> MGSSHHHHHHHSSGRENLYFQGHMEGVRWAFSCGTWLPSRAEWLLAVRSIQPEEKERIGQFVFARDAKAAMAGRLMIRKLVAEKLNIPWNHIRLQRTAKGKPVLAKDSSNPYPNFNFNISHQGDYAVLAAEPELQVGIDIMKTSFPGRGSIPEFFHIMKRKFTNKEWETIRSFKDEWTQLDMFYRNWALKESFIKAIGVGLGFELQRLEFDLSPLNLDIGQVYKETRLFLDGEEEKEWAFEESKIDEHHFVAVALRKPDGSRHQDVPSQDDSKPTQRQFTILNFNDLMSSAVPMTPEDPSFWDCFCFTEEIPIRNGTKS;> GTRDRDSQRDLVEAVAHILGIRDLAAVNLDSSLADLGLDALMSVEVRQTLERELNLVLSVREVRQLTLRKLQELSSKADEASELACPTPKE

The posttranslational modification of a conserved serine residue in carrier proteins with a phosphopantetheinyl moiety transferred from coenzyme A through the enzyme phosphopantetheinyl transferase (PPT) is vital to all living organisms. Molecular cloning and biochemical characterization of human PPT revealed that this cytosolic enzyme is a Mg2+-requiring monomeric enzyme that exhibits a broad acceptor substrate specificity. Whereas microbial genomes contain more than one PPT, only one PPT has been identified in mammals. This enzyme exhibits a broad substrate specificity and is able to phosphopantetheinylate the ACP components of the cytosolic and the mitochondrial FAS systems, as well as aminoadipate semialdehyde dehydrogenase, the human ortholog to the yeast lys5 gene. Human phosphopantetheinyl transferase exhibits an α/β fold and 2-fold pseudosymmetry similar to the Sfp phosphopantetheinyl transferase from Bacillus subtilis.

The serine acceptor residue for the phosphopantetheinyl moiety in ACP was mutated to alanine to facilitate crystallization of a stable ternary complex of PPT, apoACP, and CoA. The type I human ACP binds in the cleft between the two domains of the PPT and the essential Ser2156Ala points directly toward the β-phosphate of the bound CoA. The interaction between the two proteins takes place on a large interface and is mostly of hydrophobic character. Three hydrophobic patches on the PPT surface interact with the ACP. A few polar interactions that involve hydrogen bonds and salt bridges can be observed (ACP-PPT: Arg2138-Gly137, Asp2151-Gln50, Thr2165-Arg138, Glu2169-Arg138), but binding specificity seems to be determined by shape complementarity rather than through the few specific interactions. Upon binding the ACP, the two domains of PPT rotate around a hinge consisting of residue Glu133, and close slightly (3.9 Å at the furthest point from the hinge, or approximately 10 degrees). For the PPT-CoA-ACP complex, the packing within the crystal lattice is different, and this region is no longer visible in the electron density maps, indicating inherent flexibility. On the other hand, the position of the bound CoA is changed only slightly on binding of ACP, and the phosphopantetheine moiety is now disordered, possibly oriented away from the active site to avoid collision with the bound ACP. Surprisingly, in the PPT-CoA-ACP complex, no density was found for the Mg that is sequestered in the active center of the PPT-CoA complex. This may be explained by a water molecule that coordinates the Mg in the PPT-CoA structure, which is displaced by the Ala side chain (substituted for the Ser2156) when complexed with ACP.>MDIKVHFHDFSHVRIDCEESTFHELRDFFSFEADGYRFNPRFRYGNWDGRIRLLDYNRLLPFGLVGQIKKFCDNFGYKAWIDPQINEKEELSRKDFDEWLSKLEIYSGNKRIEPHWYQKDAVFEGLVNRRRILNLPTSAGRSLIQALLARYYLENYEGKILIIVPTTALTTQMADDFVDYRLFSHAMIKKIGGGASKDDKYKNDAPVVVGTWQTVVKQPKEWFSQFGMMMNDEC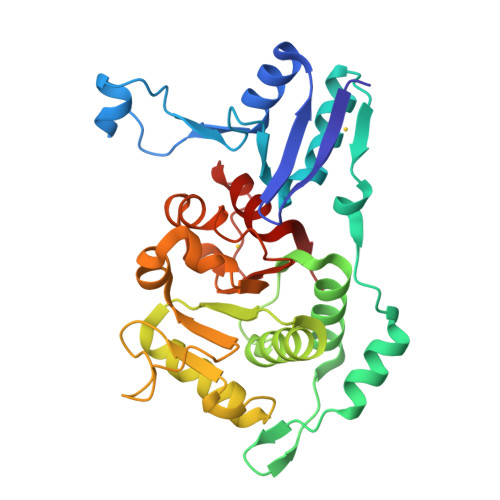HLATGKSISSIISGLNNCMFKFGLSGSLRDGKANIMQYVGMFGEIFKP[2x]> MAEGETESPGPKKSGPYISSVTSQSVNLMIRGVVLFFIGVFLALVLNLLQIQRNVTLFPPDVIASIFSSAWWVP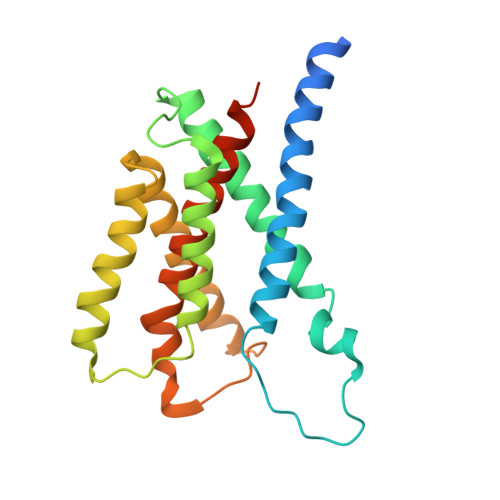PCCGTASAVIGLLYPSIDRHLGEPHKFKREWSSVMRCVAVFVGINHASAKVDFDNNIQLSLTLAALSIGLWWTFDRSRSGFGLGVGIAFLATVVTQLLVYNGVYQYTSPDFLYVRSWLPCIFFAGGITMGNIGRQLAMYESKVIAEKSHQE> AAAMEEKTIYIAGLGLIGASLALGIKRDHPHYKIVGYNRSDRSRDIALERGIVDEATADFKVFAALADVIILAVPIKKTIDFIKILADLDLKEDVIITDAGSTKYEIVRA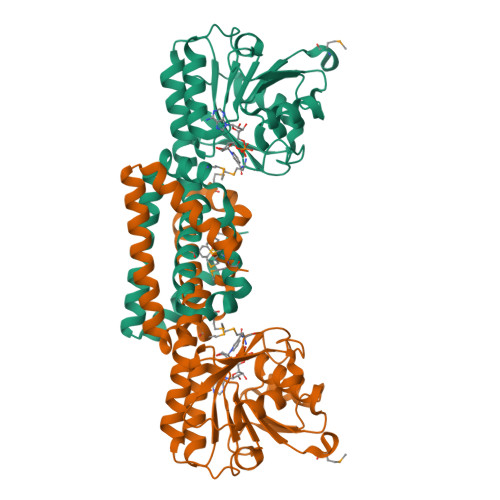AEYYLKDKPVQFVGSHPMAGSHKSGAVAANVNLFENAYYIFSPSCLTKPNTIPALQDLLSGLHARYVEIDAAEHDCVTSQISHFPHIIASSLMKQAGDFSESHEMTKHFAAGGFRDMTRIAESEPGMWTSILLTNQEAVLDRIENFKQRLDEVSNLIKARDENAIWAFFNQSRQIRKNME D-phenylalanyl-N-{4-[amino(iminio)methyl]benzyl}-L-prolinamide 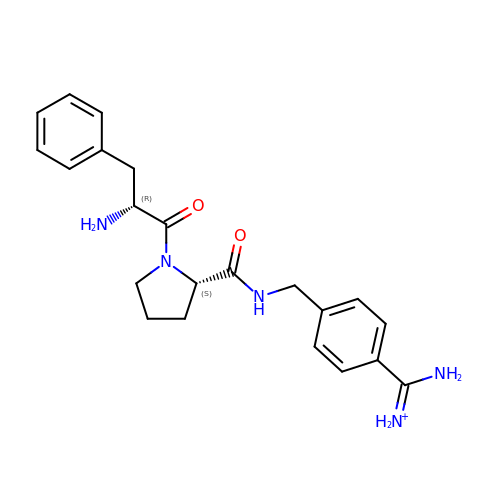| C22 H28 N5 O2 | VZFTWWJAUZOJDH-MOPGFXCFSA-O> MNQNLLVTKRDGSTERINLDKIHRVLDWAAEGLHNVSISQVELRSHIQFYDGIKTSDIHETIIKAAADLISRDAPDYQYLAARLAIFHLRKKAYGQFEPPALYDHVVKMVEMGKYDNHLLEDYTEEEFKQMDTFIDHDRDMTFSYAAVKQLEGKYLVQNRVTGEIYESAQFLYILVAACLFSNYPRETRLQYVKRFYDAVSTFKISLPTPIMSGVRTPTRQFSSCVLIECGDSLDSINATSSAIVKYVSQRAGIGINAGRIRALGSPIRGGEAF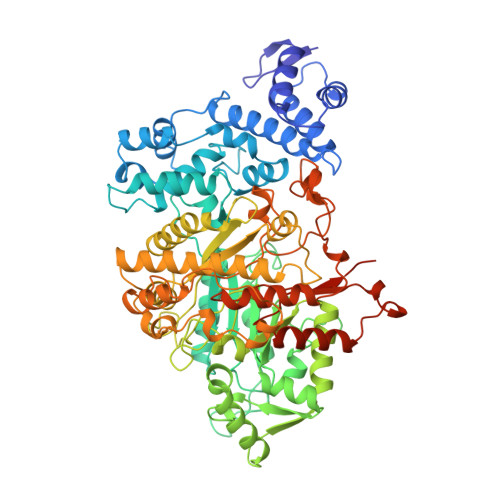HTGCIPFYKHFQTAVKSASQGGVRGGAATLFYPMWHLEVESLLVLKNNRGVEGNRVRHMDYGVQINKLMYTRLLKGEDITLFSPSDVPGLYDAFFADQEEFERLYTKYEKDDSIRKQRVKAVELFSLMMQERASTGRIYIQNVDHCNTHSPFDPAIAPVRQSNLCLEIALPTKPLNDVNDENGEIALCTLSAFNLGAINNLDELEELAILAVRALDALLDYQDYPIPAAKRGAMGRRTLGIGVINFAYYLAKHGKRYSDGSANNLTHKTFEAIQYYLLKASNELAKEQGACPWFNETTYAKGILPIDTYKKDLDTIANEPLHYDWEALRESIKTHGLRNSTLSALMPSETSSQISNATNGIEPPRGYVSIKASKDGILRQVVPDYEHLHDAYELLWEMPGNDGYLQLVGIMQKFIDQSISANTNYDPSRFPSGKVPMQQLLKDLLTAYKFGVKTLYYQNTRDGAEDAQDDLVPSIQDDGCESGACKI> SRFADAVLDQYIGSIHSLCKDQHGCRFLQKQLDILGSKAADAIFEETKDYTVELMTDSFGNYLIQKLLEEVTTEQRIVLTKISSPHFVEISLNPHGTRALQKLIECIKTDEEAQIVVDSLRPYTVQLSKDLNGNHVIQKCLQRLKPENFQFIFDAISDSCIDIATHRHGCCVLQRCLDHGTTEQCDNLCDKLLALVDKLTLDPFGNYVVQYIITK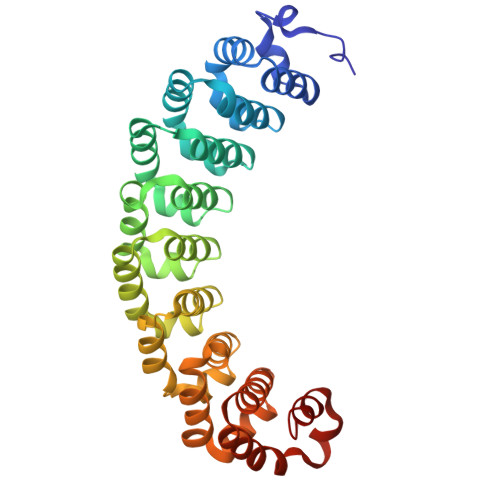EAEKNKYDYTHKIVHLLKPRAIELSIHKFGSNVIEKILKTAIVSEPMILEILNNGGETGIQSLLNDSYGNYVLQTALDISHKQNDYLYKRLSEIVAPLLVGPIRNTPHGKRIIGMLHL>MENNGIDGVVLYEDADHKFIWLGSESKQRKGAVQTMQYLIVDRGRGVLLDPGGVHLFSRVVTAISRFISVDKIDTIFFSHQDPDVSSGIALWLGITKAKIYISSLWVRFMPHFGIVDISRMVPIPDKGMSISLPSGSNMKCIPSHFMHSPGQFGLYDERSR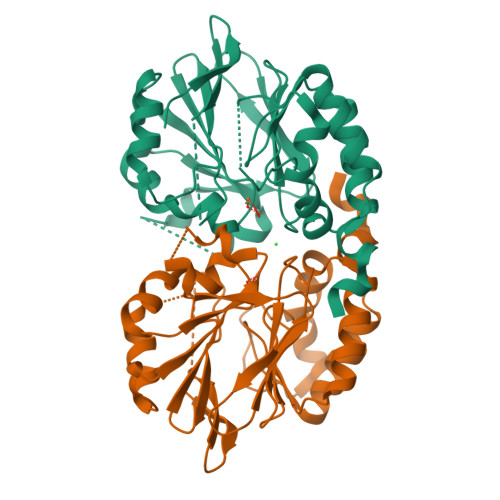ILFSGDIGAAVFDDDNETTFVEDFEKHLPLIEGFHVRYMASNKIVSKWVEYVRRLNPLMIAPQHGAIYKDEQVNNFLNWLSGLKCGTDYIENLF[2x]3-{2-[1-(5-HYDROXY-1,5-DIMETHYL-HEXYL)-7A-METHYL-OCTAHYDRO-INDEN-4-YLIDENE]-ETHYLIDENE}-4-METHYLENE-CYCLOHEXANOL | C27 H44 O2 | 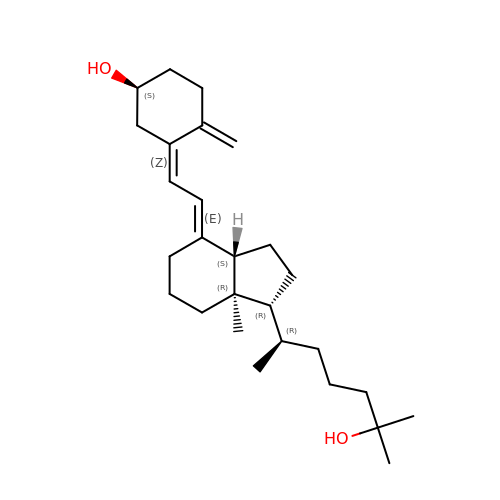JWUBBDSIWDLEOM-DTOXIADCSA-N(2R,3R,4R,5S)-2-(hydroxymethyl)oxane-2,3,4,5-tetrol | C6 H12 O6 | 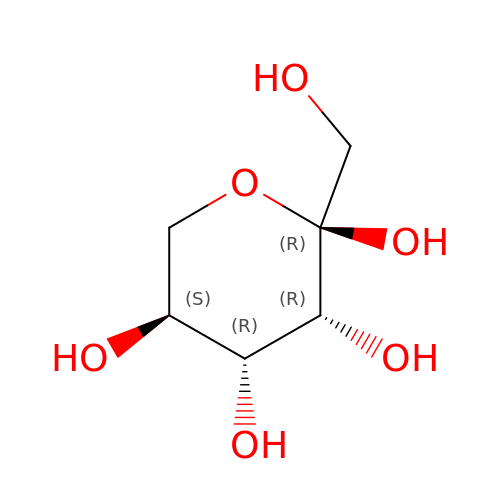LKDRXBCSQODPBY-SLPGGIOYSA-N>MDEYVQELKGLIRKHIPERCEFGHQKVTFLSQVHPSPLLTEGFKLLSSLVELESCEAHACQANTDQRFVDVILSDNGILCPTLPKVIPDGFKLTGKTLILLETFVRVNPDEFEKKWKADMSKLLNLKHDLQKSGVTLVPIVDGRSNYNNRFVADWVIERIRWLLIEILKASKSMLEIDIEDQEYQRLIHSLSNVKNQSLGLENLEHLKRNSLDYDERLNESLFIGLKGDIRESTVREELIKLKLWFKDEVFSKGLGKFKLTDRRELLESLSSLGAHLDSDVSSCPFCNNKLMEIVYNVTFSCVERTDGVATVDQQFSTTHSNIEKHYLSVLSLCNKIKGLKVFNTRRNTLLFLDLIMVNLMVDISDSCQDAIESLRKSGLIVGQMVMLVNDRVLDILEAVKLIRKKIGTNPNWVKNCSKILERSHPEIWHHLSTLIKQPDFNSLISIAQHLVSDRPIMRYSVERGSDKICRHKLFQEMSSFEQMRLFKTLSSISLSLINSMKTSFSSRLLVNEREFSKYFGNVRLRECYAQRFYLAESLVGFLFYQKTGERSRCYSVYLSDNGVMSEQGSFYCDPKRFFLPVFSDEVLAGMCEEMTSWLDFDTGLMNDTGPILRLLVLAILCSPSKRNQTFLQGLRYFLMAFANQIHHIDLTSKLVVECKSSSEVVVQRLAVGLFIRLLSGESDASLFFSRRFKYLLNVSYLCHLITKETPDRLTDQIKCFEKFIEPKVKFGCAVVNPSLNGKLTVDQEDIMINGLKKFFSKSLRDTEDVQTPGVCKELLNYCVSLFNRGKLKVSGELKNNPFRPNITSTALDLSSNKSVVIPKLDELGNILSTYDKEKLVSACVSSMAERFKTKGRYNLDPDSTDYLILKNLTGLVSAGPKAKSTQEELSLMYEALTEEQVESFNEIKHDVQVALAKMADNSVNTRTKNLGRADNSVKNGNNPLDNLWSPFGVMKEIRAEVSLHEVKDFDPDVLPPEVYKELCDAVYKSSEKCNFFLEGVLDVCPLGLLLKNLTTSSYVDEEYFMCFKYLLIQGHFDQKLGSYEHKSRSRLGFTDETLRLKDEVRLSIRESNSEAIADKLDKSYFTNAALRNLCFYSEDSPTEFTSISSNSGNLKFGLSYKEQVGSNRELYVGDLNTKLMTRLVEDFSEAVGNSMKYTCLNSEKEFERAICDMKMAVNNGDLSCSYDHSKWGPTMSPALFLALLQMLELRTPVDRSKIDLDSVKSILKWHLHKVVEVPINVAEAYCIGKLKRSLGLMGCGSTSLSEEFFHQTMQLNGQIPSHIMSVLDMGQGILHNTSDLYGLITEQFLCYALDLLYDVIPVSYTSSDDQITLIKTPSLDIEGGSDAAEWLEMICFHE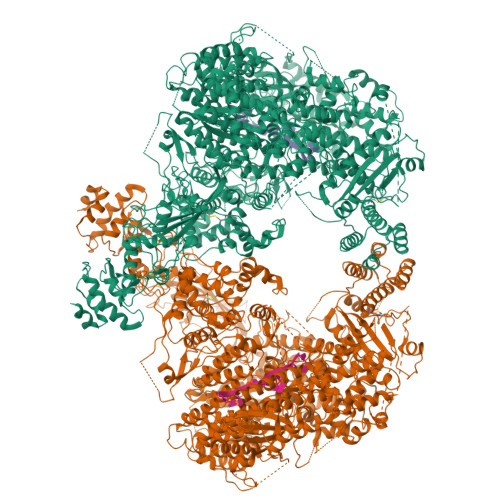FLSSKLNKFVSPKSVIGTFVAEFKSRFFVMGEETPLLTKFVAAALHNVKCKTPTQLSETIDTICDQCIANGVSTKIVTRISKRVNQLIRYSGYGETPFGAIEDQDVKDWVDGSRGYRLQRKIEAIFHDDKETSFIRNCARKVFNDIKRGRIFEENLINLIGRGGDEALTGFLQYAGCSEQEVNRVLNYRWVNLSSFGDLRLVLRTKLMTSRRVLEREEVPTLIKTLQSKLSRNFTKGVKKILAESINKSAFQSSVASGFIGFCKSMGSKCVRDGKGGFLYIKEVYSGVSACTCEICALKPKIIYCNNSLNKVSQFSKPILWDYFSLVLTNACELGEWVFSTVKEPQKPLVLNNQNFFWAVKPKVVRQIEDQLGMNHVLQSIRRNYPVLFDEHLTPFMNDLQVSRTMDSGRLKFLDVCIALDMMNENLGIISHLLKTRDNSVYIVKQSDCALAHIRQSSYTDWELGLSPQQICTNFKTQLVLSSMVNPLVLSTSCLKSFFWFNEVLELEDDSQIELAELTDFALMVKNQNVSRAMFVEDIAMGYVVSNFEGVRISLSNVMVDGVQLPPQEKAPDIGELFGLKAENVIVGLVVQIDHVRMSTKFKLKRKMVYSFSLECIMDVGEIQNKEVILKVVAVDQSVSGSGGNHMLLDGVSVVASLPLFTGQASFDLAAMLIESNLAGSNDNFLMRNVTLDLGGFSPELSDKYSYRLSGPENQEDPLVLKDGAFYVGGERLSTYKVEFTGDLVVKALGALEDDESVVSMLHQLWPYLKATSQVILFQQEDFTIVHDLYKKQLTKSIESFGEWIEFTNFKVAYSKSLKELVISDTQGSFRLKGVMCRPLASTPQVEDIE[2x]> GAQVSRQNVGTHSTQNMVSNGSSINYFNINYFKDAASSGASR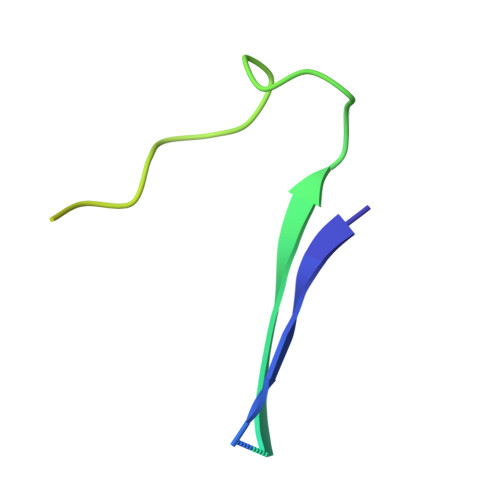LDFSQDPSKFTDPVKDVLEKGIPTLQSPSVEACGY> MSMTPDLAGLFEGASTYPDVDARERLNNLVGLDTHKSRLSKMLAVLVNPDGLSAWAKKHHPAAEALVKNVIRRPPLIVLAGDVGSGKTELA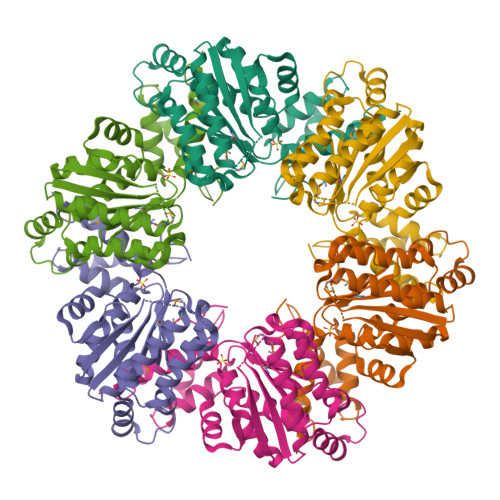ETIGDDVARRESIRITLLPLSLSARGQGRVGEMTQLISAAFEHTVSEARKLKSSGTKARGAVILLVDEADALAQSREAAQMHHEDRAGVNAFIRGIDRLGNGALPAAVIMCTNRVDSLDPAVRRRAAEIITFDRPNDAQRRAVITTTLQGTGVTGSQIEGLVAATGPARPRDYGFTFSDLTQRLIPSIVLDAYPDTSINPARALAIAQAMAPTAPFQDKSR>METTDTKREEQEIEEKKAQEESKIEDVDKILNDILSISSECIQPDELRVKLLLKRKLICYDGFEPSGRMHIAQGLLKSIIVNKLTSNGCTFIFWIADWFAHLNNKMSGDLKKIKKVGSYFIEVWKSCGMNMENVQFLWASEEINKKPNEYWSLVLDISRSFNINRMKRCLKIMGRSEGEENYCSQILYPCMQCADIFFLNVDICQLGIDQRKVNMLAREYCDIKKIKKKPVILSHGMLPGLLEGQEKMSKSDENSAIFMDDSESDVNRKIKKAYCPPNVIENNPIYAYAKSIIFPSYNEFNLVRKEKNGGDKTYYTLQELEHDYVNGFIHPLDLKDNVAMYINKLLQPVRDHFQNNIEAKNLLNEIKKYKVTK[2x]

The Plasmodium falciparum cytoplasmic tyrosine tRNA synthetase (PfTyrRS) is an attractive drug target that is susceptible to reaction-hijacking by AMP-mimicking nucleoside sulfamates. PfTyrRS is a Class I aaRS, characterized by a catalytic domain with a Rossmann fold (residues 18–260) linked to a C-terminal anti-codon binding domain (residues 261–370) involved in recognition of tRNATyr. PfTyrRS contains “HIGH” and “KMSKS” (70HIAQ74 and 247KMSKS251 in PfTyrRS) motifs that are characteristic of the catalytic domain of Class I tRNA synthetases (sub-class c). ML901 binds the P. falciparum cytoplasmic tyrosine tRNA synthetase (PfTyrRS), and then reacts with the bound activated amino acid, resulting in the synthesis of an inhibitory sulfamate-amino acid adduct within the active site of the enzyme.

We confirm that ML471 is a reaction hijacking inhibitor that is converted into a tight binding Tyr-ML471 conjugate by the PfTyrRS enzyme. The complex of PfTyrRS with synthetic Tyr-ML471 was crystalised using previously established conditions and the structure refined at 1.8 Å resolution, revealing a homodimer organization with clear density for the Tyr-ML471 ligand. Tyr-ML471 makes many interactions with active site residues, involving the pyrazolopyrimidine amine, ribose hydroxyls, sulfamate, and tyrosine. The 7-position isopropyl group is oriented away from the binding pocket and is partially solvent exposed, consistent with the docking study. The isopropyl group of ML471 is oriented differently in the A- and B-chains and the adjacent His70 (of 70HIAQ73) adopts different side chain rotamers in each chain. The majority of the KMSKS loop was poorly defined in the electron density in both chains, suggesting flexibility. By contrast the isopropyl group of ML471 in chain B is oriented with one methyl group towards His70 (blue arrow), and the His70 side chain adopts a rotamer that is incompatible with the Met248 interaction observed for Tyr-ML901. Thus, for chain B, Tyr-ML471 binding appears to be associated with loop destabilisation while Tyr-ML901 binding is associated with loop stabilisation. The pose adopted by the 7-position isopropyl group of ML471 appears to re-position His70, leading to increased flexibility of the KMSKS loop. This may, in turn, enhance the binding or re-binding of the Tyr-tRNA product, positioning the Tyr-tRNA carbonyl carbon for attack by the sulfamate nitrogen of ML471.> MKQYLELMQKVLDEGTQKNDRTGTGTLSIFGHQMRFNLQDGFPLVTTKRCHLRSIIHELLWFLQGDTNIAYLHENNVTIWDEWADENGDLGPVYGKQWRAWPTPDGRHIDQITTVLNQLKNDPDSRRIIVSAWNVGELDKMALAPCHAFFQFYV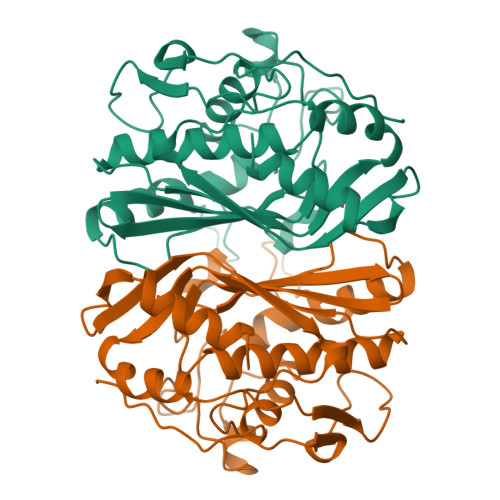ADGKLSCQLYQRSCDVFLGLPFAIASYALLVHMMAQQCDLEVGDFVWTGGDTHLYSNHMDQTHLQLSREPRPLPKLIIKRKPESIFDYRFEDFEIEGYDPHPGIKAPVAI>AKVLVLYYSMYGHIETMARAVAEGASKVDGAEVVVKRVPETMPPQLFEKAGGKTQTAPVATPQELADYDAIIFGTPTRFGNMSGQMRTFLDQTGGLWASGALYGKLASVFSSTGTGGGQEQTITSTWTTLAHHGMVIVPIGYAAQELFDVSQVRGGTPYG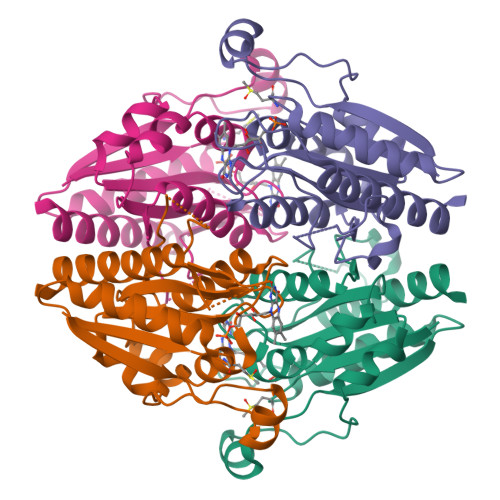ATTIAGGDGSRQPSQEELSIARYQGEYVAGLAVKLNG[2x]> MVLLESEQFLTELTRLFQKCRTSGSVYITLKKYDGRTKPI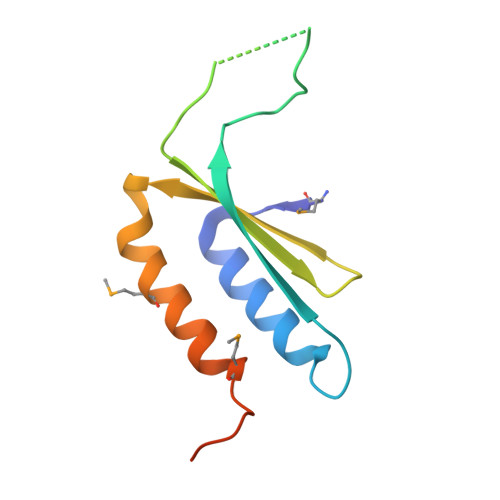PKKGTVEGFEPADNKCLLRATDGKKKISTVVSSKEVNKFQMAYSNLLRANMDGLKKRDKKNKTKKTK>[4x]MAAASTAKIVIIGSYNRDLVWYVKDFPI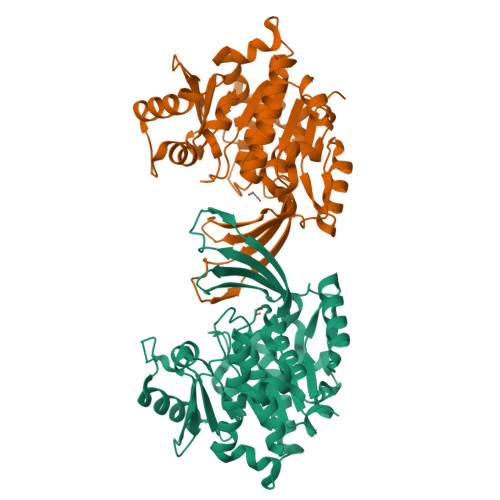GGQTINGSFASSHGGKGSNQAIACGKVLRDPSRAFFVGAVGKDTFGDEILAHYRELGIPNCIKQVSGAPTGNAGIYVAESGENMIVISEGANGMLKPSLVPDLMAVLVKATLVVMQCEISPDNTLLFVEVIKQAKAQNSSLRFVFNPAPYRADYDFSKILSITDIFCPNELEALEISGTGRLEGICDDSMMKALVEKMSSLSPSLKFVLFTLGSRGSRIVQTKSYESRTVGIYSHGRAIDTSGAGDCFIGSFCVRLMELAEESTRGPSALNDIDTIAEAARFASVAAGISVTRKGTSASVPRRQEVDDALSKFSGKGHHHHHH>[6x]VGALAVV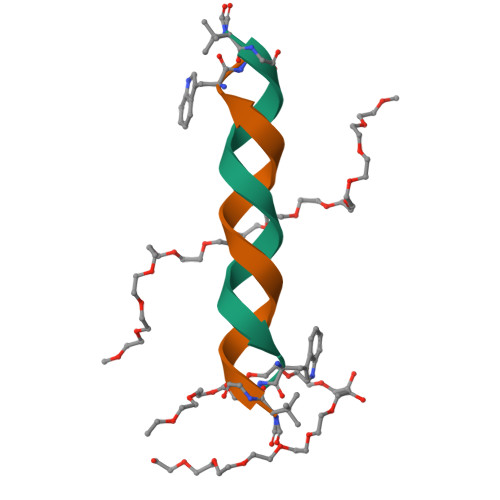VWLWLWLWX> MLDINAFLVEKGGDPEIIKASQKKRGDSVELVDEIIAEYKEWVKLRFDLDEHNKKLNSVQKEIGKRFKAKEDAKDLIAEKEKLSNEKKEIIEKEAEADKNLRSKINQVGNIVHESVVDSQDEENNELVRTWTPENYKKPEQIAAATGAPAKLSHHEVLLRLDGYDPERGVRIVGHRGYFLRNYGVFLNQALINYGLSFLSSKGYVPLQAPVMMNKEVMAKTAQLSQFDEELYKVIDGEDEKYLIATSEQPISAYHAGEWFESPAEQLPVRYAGYSSCFRREAGSHGKDAWGIFRVHAFEKIEQFVLTEPEKSWEEFDRMIGCSEEFYQSLGLPYRVVGIVSGELNNAAAKKYDLEAWFPFQQEYKELVS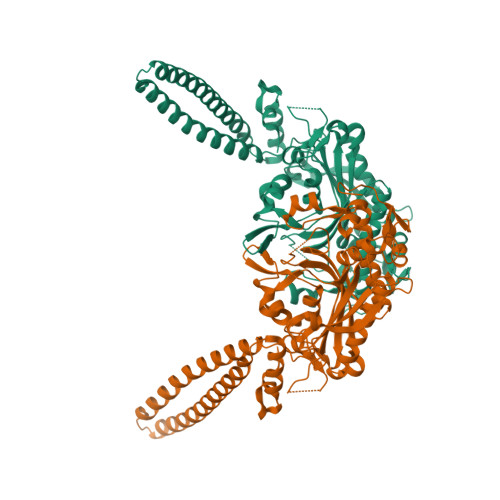CSNCTDYQSRNLEIRCGIKQQNQQEKKYVHCLNSTLSATERTICCILENYQKEDGLVIPEVLRKYIPGEPEFIPYIKELPKNTTSVKKAKGKNPKNTTSVKKAKGKNGSRHHHHHH> MKHHHHHHPMAWFPESMRQQLSGIFAKLTKKVTLLQFLDASDEKSLELQSFLTEFASLDQKITLETILKDTEPAKELLYGIEKMPSVVLLDA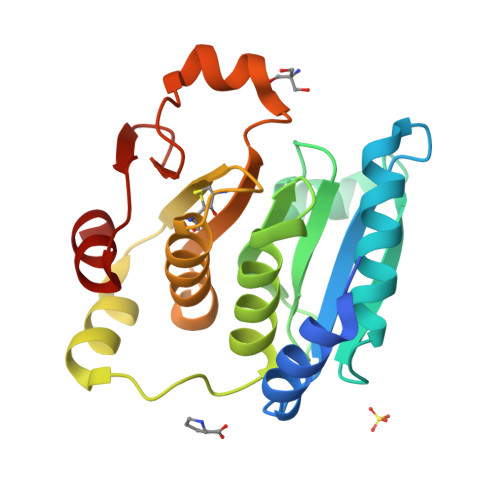AGNYTGIKFSGIPSGHEVNSLVLAVYNVGSEGQPLEASLQKNILALPKRKIEIFVSLTCHFCPDVVAACQRIASINPHVEAEMVDISLFPELKKEKKIMSVPAMLIDGEQMIFGSKTMTEIIEALA> TSSANEDMPVERILEAELAVEPKTETYVEANMGLNPSSPNDPVTNICQAADKQLFTLVEWAKRIP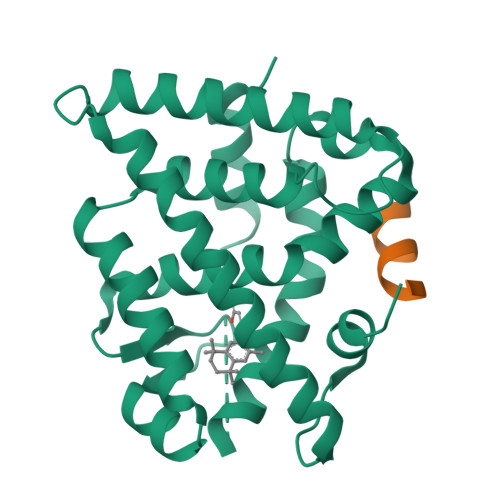HFSELPLDDQVILLRAGWNELLIASFSHRSIAVKDGILLATGLHVHRNSAHSAGVGAIFDRVLTELVSKMRDMQMDKTELGCLRAIVLFNPDSKGLSNPAEVEALREKVYASLEAYCKHKYPEQPGRFAKLLLRLPALRSIGLKCLEHLFFFKLIGDTPIDTFLMEMLEAPHQMT;> KHKILHRLLQASS>[2x]MAHTAAERPPEETLSLWKGEQARLKARVVDRDTEAWQRDPSFSGLQKVGGVDVSFVKGDSVRACASLVVLSYPELKVVYEDSRMVGLKAPYVSGFLAFREVPFLVELVQRLQEKEPDLMPQVVLVDGNGVLHQRGFGVACHLGVLTELPCIGVAMKLLQVDGLENNALHKEKIVLLQAGGDTFPLIGSSGTVLGMALRSHDHSTKPLYVSVGHRISLEVAVRLTHHCCRFRIPEPIRQA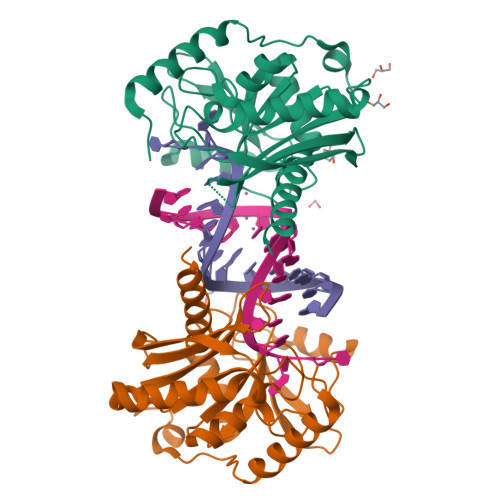DIRSREYIRRTLGQ3-(carboxymethyl)-5,7-dichloro-1H-indole-2-carboxylic 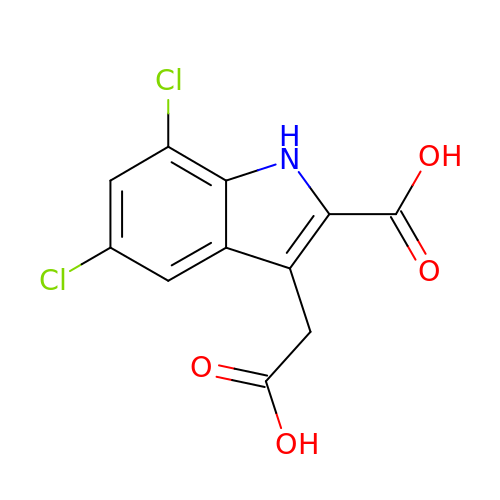acid | C11 H7 Cl2 N O4 | UDTYSEWCICAFSB-UHFFFAOYSA-N The levels of MepS are regulated via proteolysis by a newly identified protease complex consisting of Prc, a soluble periplasmic PDZ-protease (also known as tail-specific protease, Tsp), and NlpI, an OM lipoprotein with tetratricopeptide repeats (TPRs). NlpI serves as an adaptor protein that binds Prc to target MepS for degradation; however, interestingly, the latter two do not interact with each other. Prc belongs to the large family of C-terminal processing proteases that recognize the C terminus of protein substrates. The lipoprotein NlpI has the dual role of bringing the soluble periplasmic protease Prc to the OM, where the lipid-anchored substrate MepS resides, and enhancing the efficiency of MepS degradation by Prc.

We determined the crystal structure of NlpI in complex with catalytically inactive Prc-K477A (hereafter termed the sNlpI-Prc complex), at 2.30 Å resolution. The asymmetric unit (ASU) contains two NlpI molecules forming a butterfly-shaped homodimer and two circular Prc molecules binding to each side of the symmetric NlpI dimer, which are angled away from the OM. The NlpI dimer interface involves mainly the swapped N-terminal helix h0 and a 10-residue linker to helix h1. NlpI binds to Prc mainly through the TPR2b helix, which contains four exposed acidic residues (D113, E117, D120, and E124) engaging in extensive electrostatic interactions with Prc. Helix h1 makes electrostatic interactions with the TPR2b acidic residues of NlpI via basic residues R47, R51, and R484, while M493 and L494 of helix h14 make hydrophobic contacts with TPR1b–TPR2a of NlpI. The extended N-terminal and C-terminal helical domains (NHD and CHD, respectively), which associate through a pair of anti-parallel β-strands b1–b22, forms a bowl-like structure with the protease module comprising a vault and the platform domain. The lid-like PDZ domain is attached to the bowl through a double hinge, consisting of two loops with conserved hydrophobic hinge residues L245 and L340, which are connected to the vault helix h9 and the five-stranded β-sheet of the platform, respectively. A conserved open substrate-binding passage containing the proteolytic site, as seen in the structure of active CtpB6, is located to the side of the bowl near the hinged PDZ domain and is formed between the vault helix h9 and strands b2–b19–b20, and three parallel loops from the platform, which harbor the catalytic K477-S452 dyad. A co-purified peptide is bound to the proteolytic site and co-crystallized serendipitously; the unidentified peptide is modeled as poly-Ala. An unidentified peptide is also bound to the peptide-binding site of the PDZ domain in each of the two Prc molecules. Interestingly, the peptide bound to one of the PDZ domains could be tentatively modeled based on the electron-density map with the sequence LSRS-COOH, corresponding to the C-terminal four residues of MepS.

>[2x]GHMSNTSWRKSEVLAVPLQPTLQQEVILARMEQILASRALTDDERAQLLYERGVLYDSLGLRALARNDFSQALAIRPDMPEVFNYLGIYLTQAGNFDAAYEAFDSVLELDPTYNYAHLNRGIALYYGGRDKLAQDDLLAFYQDDPNDPFRSLWLYLAEQKLDEKQAKEVLKQHFEKSDKEQWGWNIVEFYLGNISEQTLMERLKADATDNTSLAEHLSETNFYLGKYYLSLGDLDSATALFKLAVANNVHNFVEHRYALLELSLLGQDQDDLAESDQQ;>MNMFFRLTALAGLLAIAGQTFAVEDITRADQIPVLKEETQHATVSERVTSRFTRSHYRQFDLDQAFSAKIFDRYLNLLDYSHNVLLASDVEQFAKKKTELGDELRSGKLDVFYDLYNLAQKRRFERYQYALSVLEKPMDFTGNDTYNLDRSKAPWPKNEAELNALWDSKVKFDELSLKLTGKTDKEIRETLTRRYKFAIRRLAQTNSEDVFSLAMTAFAREIDPHTNYLSPRNTEQFNTEMSLSLEGIGAVLQMDDDYTVINSMVAGGPAAKSKAISVGDKIVGVGQTGKPMVDVIGWRLDDVVALIKGPKGSKVRLEILPAGKGTKTRTVTLTRERIRLEDRAVKMSVKTVGKEKVGVLDIPGFYVGLTDDVKVQLQKLEKQNVSSVIIDLRSNGGGALTEAVSLSGLFIPAGPIVQVRDNNGKVREDSDTDGQVFYKGPLVVLVDRFSASASEIFAAAMQDYGRALVVGEPTFGAGTVQQYRSLNRIYDQMLRPEWPALGSVQYTIQKFYRVNGGSTQRKGVTPDIIMPTGNEETETGEKFEDNALPWDSIDAATYVKSGDLTAFEPELLKEHNARIAKDPEFQNIMKDIARFNAMKDKRNIVSLNYAVREKENNEDDATRLARLNERFKREGKPELKKLDDLPKDYQEPDPYLDETVNIALDLAKLEKARPAEQPAPVK[2x];> AAAA;>[2x]AAAAAA;> LSRS> GHMAKVKNLTKAAKPGKAAVSGDFSDSYKHNTASRLSQSVDGEMFQTRNVDFKAKSIGTKIHD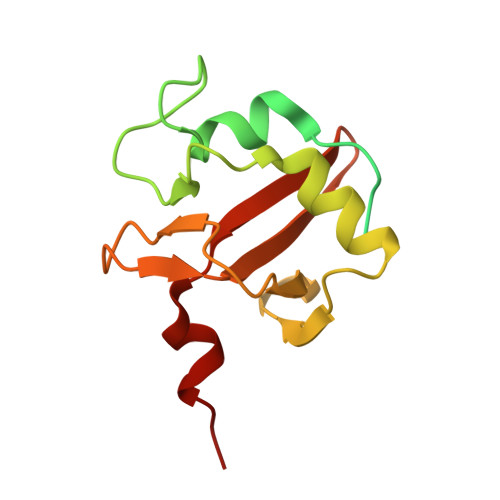GAQGKHISGHRNYIEGKSTLNQNINPQELLNGIHSGAYPVISKGARRNPVVDFGYPIGSDGKSGLSTNFGTIHSGKNGVHIVPANPKTIKKVQLE> MTAPILLLDGASMWFRSYFGVPSSIKAPDGRPVNAVRGFIDAISTLVTREKPRRLVVCRDDDWRPQWRVDLIPSYKAHRVAEPEPDGVPDIEEVPDDLTPQVNMILELLDAFGIPTAGAAGFEANDVLGTLSAREERDPVVVVSGDRDLLQLVRDEPAPQVRVLYLGRGLAKATKWGPAEVAEQYGVPLD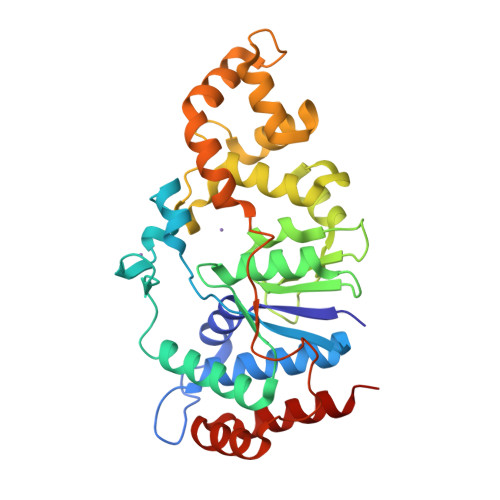RAGTAYAELALLRGDPSDGLPGVAGIGEKTAASLLAKHGSLQNILDAAHDPKSGLSKAHRTKLLGAVDYIAAAETVVRVATDAPVTFSTPTDTLPLAAGDPARVAELAAAYGVSSSISRLQTALDQLPD>[2x]MH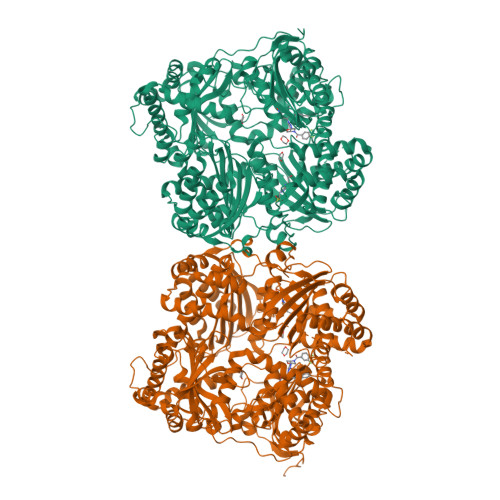HHHHHAAGIPMNNPAIKRIGNHITKSPEDKREYRGLELANGIKVLLISDPTTDKSSAALDVHIGSLSDPPNIAGLSHFLEHMLFLGTKKYPKENEYSQFLSEHAGSSNAFTSGEHTNYYFDVSHEHLEGALDRFAQFFLSPLFDESAKDREVNAVDSEHEKNVMNDAWRLFQLEKATGNPKHPFSKFGTGNKYTLETRPNQEGIDVRQELLKFHSAYYSSNLMAVVVLGRESLDDLTNLVVKLFSEVENKNVPLPEFPEHPFQEEHLKQLYKIVPIKDIRNLYVTFPIPDLQKYYKSNPGHYLGHLIGHEGPGSLLSELKSKGWVNTLVGGQKEGARGFMFFIINVDLTEEGLLHVEDIILHMFQYIQKLRAEGPQEWVFQELKDLNAVAFRFKDKERPRGYTSKIAGILHYYPLEEVLTAEYLLEEFRPDLIEMVLDKLRPENVRVAIVSKSFEGKTDRTEEWYGTQYKQEAIPDEVIKKWQNADLNGKFKLPTKNEFIPTNFEILPLEKEATPYPALIKDTAMSKLWFKQDDKFFLPKANLNFEFFSPFAYVDPLHSNMAYLYLELLKDSLNEYAYAAELAGLSYDLQNTIYGMYLSVKGYNDKQPILLKKIIEKMATFEIDEKRFEIIKEAYMRSLNNFRAEQPHQHAMYYLRLLMTEVAWTKDELKEALDDVTLPRLKAFIPQLLSRLHIEALLHGNITKQAALGIMQMVEDTLIEHAHTKPLLPSQLVRYREVQLPDRGWFVYQQRNEVHNNSGIEIYYQTDMQSTSENMFLELFAQIISEPAFNTLRTKEQLGYIVFSGPRRANGIQGLRFIIQSEKPPHYLESRVEAFLITMEKSIEDMTEEAFQKHIQALAIRRLDKPKKLSAESAKYWGEIISQQYNFDRDNTEVAYLKTLTKEDIIKFYKEMLAVDAPRRHKVSVHVLAREMDSNPVVGEFPAQNDINLSQAPALPQPEVIQNMTEFKRGLPLFPLVKPHINFMAAKL> GSRSEPAKVVDIRIDTSAERKPISPYIYGSNQELDATVTAKRFGGNRTTGYNWENNFSNAGSDWLHYSDTYLLEDGGVPKGEWSTPASVVTTFHDKALSKNVPYTLITLQAAGYVSADGNGPVSQEETAPSSRWKEVKFEKGAPFSLTPDTEDDYVYMDEFVNYLVNKYGNASTPTGIKGYSIDNEPALWSHTHPRIHPDNVTAKELIEKSVALSKAVKKVDPYAEIFGPALYGFAAYETLQSAPDWGTEGEGYRWFIDYYLDKMKKASDEEGKRLLDVLDVHWYPEARGGGERICFGADPRNIETNKA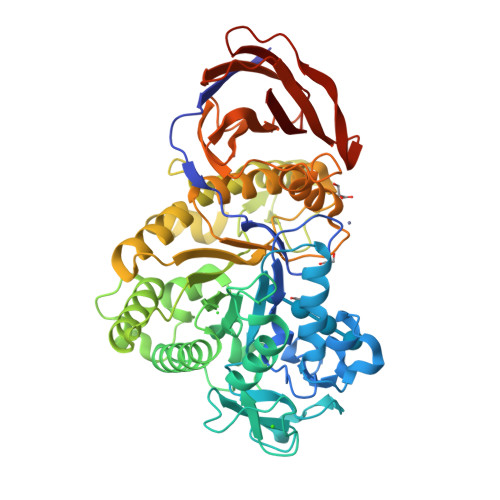RLQAPRTLWDPTYIEDSWIGQWKKDFLPILPNLLDSIEKYYPGTKLAITEYDYGGGNHITGGIAQADVLGIFGKYGVYLATFWGDASNNYTEAGINLYTNYDGKGGKFGDTSVKCETSDIEVSSAYASIVGEDDSKLHIILLNKNYDQPTTFNFSIDSSKNYTIGNVWAFDRGSSNITQRTPIVNIKDNTFTYTVPALTACHIVLEAAEP>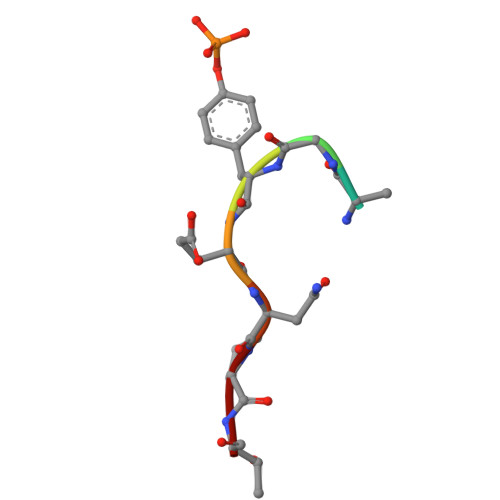 QNGYENPT> MGSSHHHHHHGSERLAFKMKLNKGQKQAYKERHDQLWPELKQLLKDNGVSEYSIFIDEETNTLFAFQKVSGHGGSQDLANN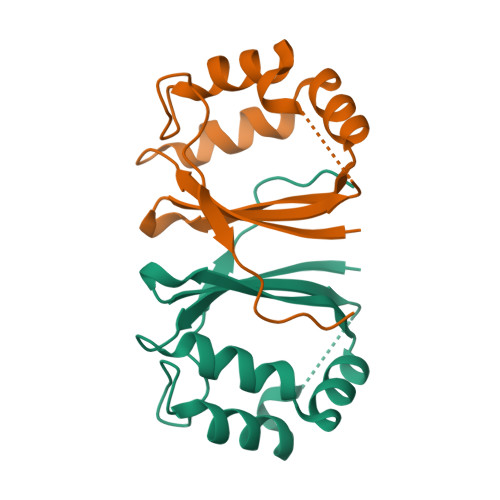EIVKKWWDFMADIMQVNPDNSPVSIPLEEVFYME> GPHMGSRSRLLAANAAAAAFYAQALQSDEAAPARQYLTERSFDAAAARKFGCGFAPSGWDSLTKHLQRKGFEFEELEAAGLSRQGRHGPMDRFHRRLLWPIRTSAGEVVGFGARRLFDDDAMEAKYVNTPETLLYKKSSVMFGIDLAKRDIAKGHQAVVVEGYTDVMAMHLAGVTTAVASCGTAFGGEHLAMLRRLMMDDSFFRGELIYVFDGDEAGRAAALKAFDGEQKLAGQSFVAVAPDGMDPCDLRLKCGDAALRDLVARRTPLFEFAIRAAIAEMDLDSAEGRVAAL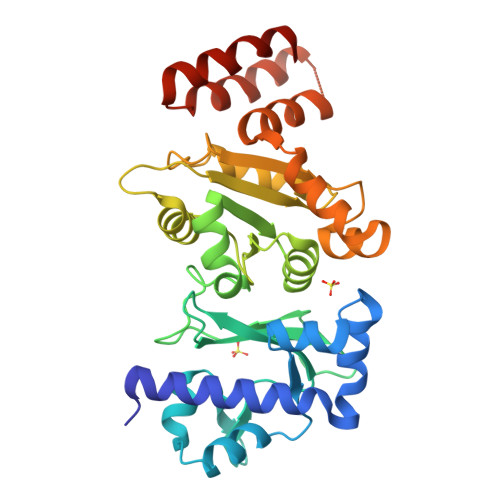RRCVPMVGQIKDPTLRDEYARQLAGWVGWADVA> MGSSHHHHHHSQDPNSMGKLTLLLLAILVWLQYSLWFGK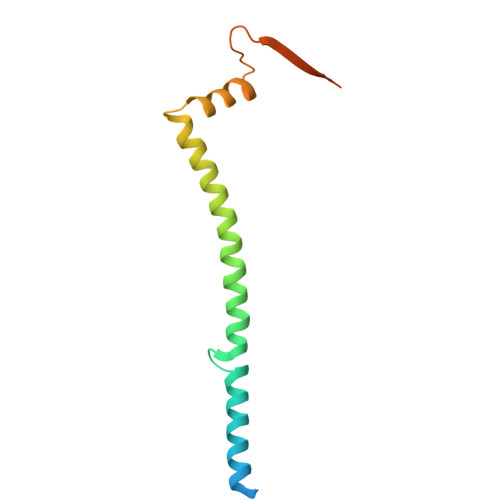NGIHDYTRVNDDVAAQQATNAKLKARNDQLFAEIDDLNGGQEALEERARNELSMTRPGETFYRLVPDASKRAQSAGQNNR> MARTAEYSIKGYLYQFLKYLSEILAAGDGARITIEGAIEDVDVIAAGLTTAVQCKYHEQAEKYTLGKIYKPILLMLEHFSKNSGTDLHVSYRLFCHFPGESGTKALTKDDLETVLSTKGEVLRAIVARIDTSVDYEAFLDRFAIEFGPSAEDLQVAVLASLKDKGFDPDDIDAVIFPNAIQRIVDLATRSDVNDRTVEPKTFLAGLREVRRVTFTRWTRELATKGRMFSSLRKSLRSCLAHNSRWRVFVINPLTIENFDDDIVRFIK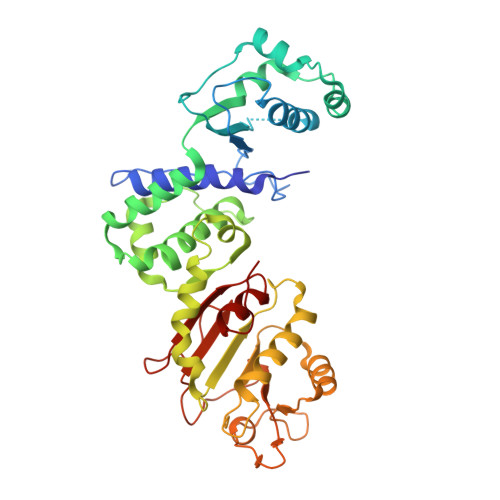AFVQRYSSKYLHSNPPLFMLTGDYDLSVLQKRLYDAGLRCETGKVGGTDVIIKELFRRPILIRNPFRMEFSLRLAKRDEVIGGPQRRPDELFLINVADDEWKHEDVNVHGFKIERLSDLEYILQLRSDYA>GPKNLQEARRKGRMDRSKAEEEMSNELQNLDVQGKSKATGTGLVYVDAFTRFHCLWDASHPECPARVSTVMEMLETEGLLGRCVQVEARAVTEDELLLVHTKEYVELMKSTQNMTEEELKTLAEKYDSVYLHPGFFSSACLSVGSVLQLVDKVMTSQLRNGFSINRPPGHHAQADKMNGFCMFNNLAIAARYAQKRHRVQRVLIVDWDVHHGQGIQYIFEEDPSVLYFSVHRYEDGSFWPHLKESDSSSVGSGAGQGYNINLPWNKVGMESGDYITAFQQLLLPVAYEFQPQLVLVAAGFDAVIGDPKGGMQVSPECFSILTHMLKGVAQGRLV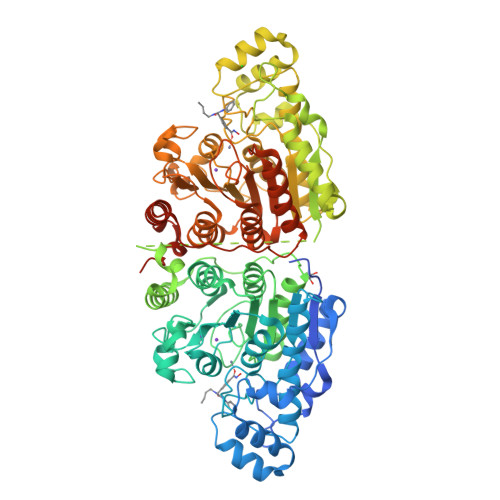LALEGGYNLQSTAEGVCASMRSLLGDPCPHLPSSGAPCESALKSISKTISDLYPFWKSLQTFEGGPLSEVSPLPAPVCAEVKVSSPITGLVYDQRMMLHHNMWDSHHPELPQRISRIFSRHEELRLLSRCHRIPARLATEEELALCHSSKHISIIKSSEHMKPRDLNRLGDEYNSIFISNESYTCALLAAGSCFNSAQAILTGQVRNAVAIVRPPGHHAEKDTACGFCFFNTAALTARYAQSITRESLRVLIVDWDVHHGNGTQHIFEEDDSVLYISLHRYEDGAFFPNSEDANYDKVGLGKGRGYNVNIPWNGGKMGDPEYMAAFHHLVMPIAREFAPELVLVSAGFDAARGDPLGGFQVTPEGYAHLTHQLMSLAAGRVLIILEGGYNLTSISESMSMCTSMLLGDSPPSLDHLTPLKTSATVSINNVLRAHAPFWSSLRVNIPESLRLSLPSPKPKGKCTPGGKGKKSPRQS[2x]> GQRWELALGRF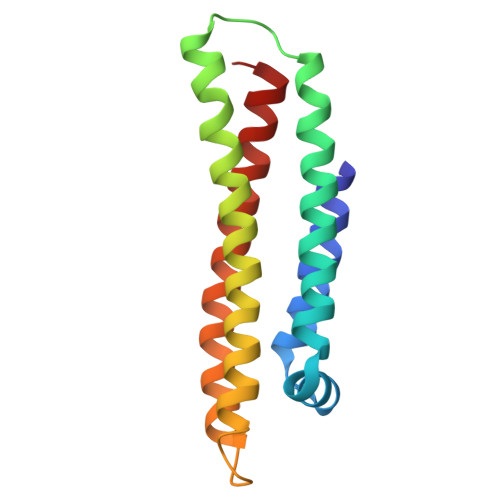WDYLRWVQTLSEQVQEELLSSQVTQELRALMDETMKELKAYKSELEEQLTPVAEETRARLSKELQAAQARLGADMEDVCGRLVQYRGEVQAMLGQSTEELRVRLASHLRKLRKRLLRDADDLQKCLAVYQAGA>[6x]AGVKTQPVAVRFALVADGKEVGCGAPLANLGSGRLAGKLHEARLYVYGFELVDAKGKHTPIALTQNDWQYADVALLDFKDARGGNAACTPGNPAKNTTVVGAAPQGAYVGLAFSVGAPVESLVDGKPVFVNHSNVEAAPPPLDISGMAW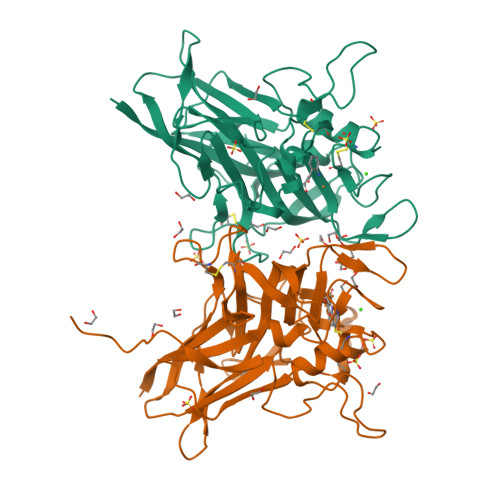NWQAGRRFVTIEVIPPAAVIKPDGSKSRTWMVHVGSTGCKGNPATGEIVACAHENRFPVVFDRFDPKTQRVELDLTTLFESSDISVDKGGAVGCMSALDDPDCPAVFRALGLNLADSAPGANDAGKPSRPGVSPIFSVGAAASKVAGGKQ>MRPLVIILMGSSSDMGHAEKIASELK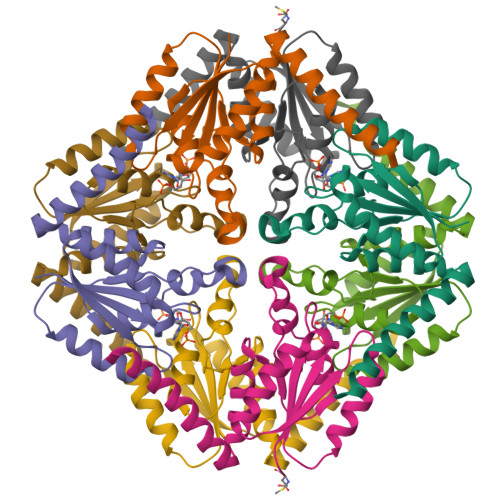TFGIEYAIRIGSAHKTAEHVVSMLKEYEALDRPKLYITIAGRSNALSGFVDGFVKGATIACPPPSDSFAGADIYSSLRMPSGISPALVLEPKNAALLAARIFSLYDKEIADSVKSYMESNAQKIIEDDSKLKR[4x]> IGWRREGIKYRRNELFLDVLESVNLLMSPQGQVLSAHVSGRVVMKSYLSGMPECKFGMNDKIVIEKQGKGTADETSKSMEQKLISEEDLGKQSIAIDDCTFHQCVRLSKFDSERSISFIPPDGEFELMRYRTTKDIILPFRVIPLVREVGRTKLEVKVVIKSNFKPSLLAQKIEVRIPTPLNTSGVQVICMKGKAKYKASENAIVWKIKRMAGMKESQISAEI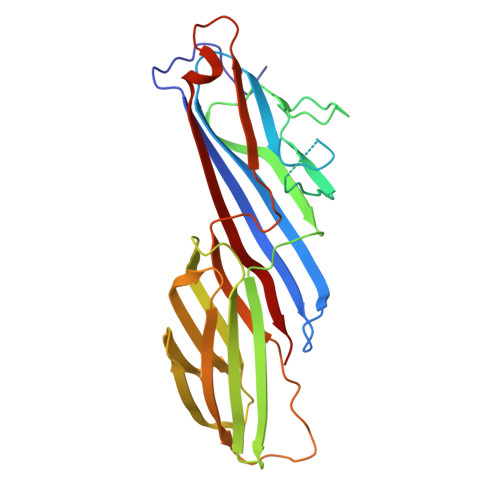ELLPTNDKKKWARPPISMNFEVPFAPSGLKVRYLKVFEPKLNYSDHDVIKWVRYIGRSGIYETRC>[4x]CDKTVEVVKNAIETADGALDLYNKYLDQVIPWQTFDETIKELSRFKQEYSQAASVLVGDIKTLLMDSQDKYFEATQTVYEWAGVATQLLAAYILLFDEYNEKKASAQKDILIKVLDDGITKLNEAQKSLLVSSQSFNNASGKLLALDSQLTNDFSEKSSYFQSQVDKIRKEAYAGAAAGVVAGPFGLIISYSIAAGVVEGKLIPELKNKLKSVQNFFTTLSNTVKQANKD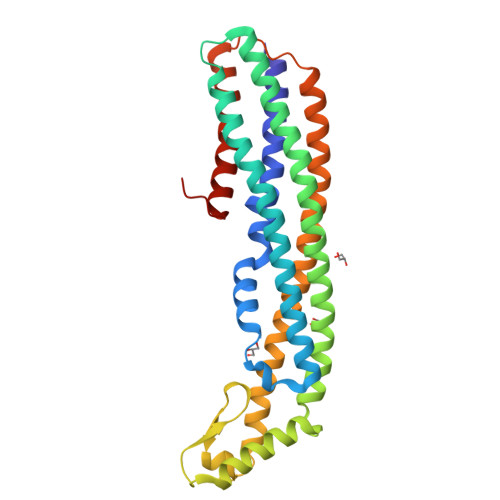IDAAKLKLTTEIAAIGEIKTETETTRFYCDYDDLMLSLLKEAAKKMINTANEYQKRHGKKTLFEVPEV2-hydroxy-4-(4-methyl-1,3-dioxo-1,3-dihydro-2H-isoindol-2-yl)benzoic acid | 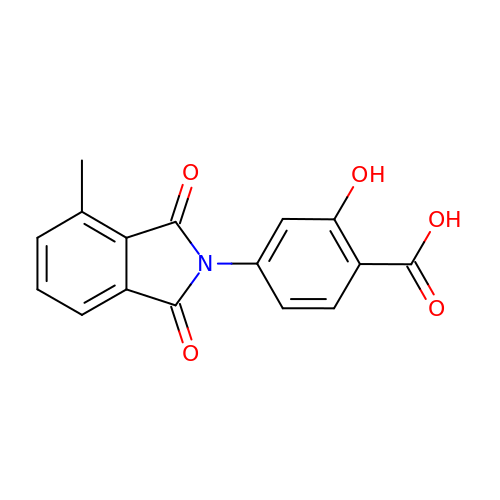C16 H11 N O5 | SPKSOWKQTVDRTK-UHFFFAOYSA-N>GPLGSNRKRLPSYLKPGSAVEIS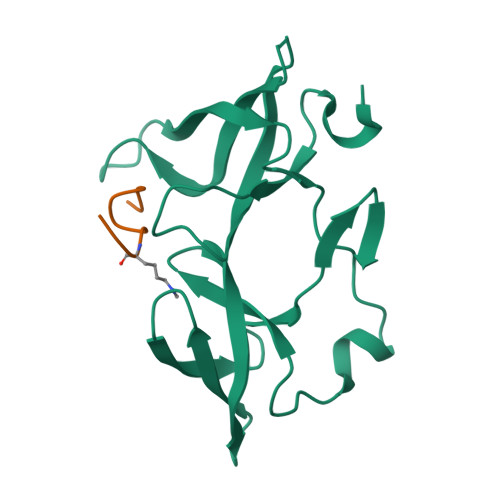SDEIGFRGSWYMGKVITIPSSSDKDSVKCQVEYTTLFFDKEGTKPLKEVVDMSQLRPPAPPMSEIEKKKKIVVGEEVDAFYNDGWWEGDVTEVLDDGKFSVFFRSSKEQIRFRKDELRFHREWVDGAWK[2x];>[2x]ARTKQTARKST> MKNPSFDWERLKDVFYRSRAIGELKWPTQYEEFKCALSLTVIAVEIQDFIQVYNYFGQLLGKINLQRIHEDIIKFEFDKDEKLILVTKSSIKIVKGWSPLTIESVPLQDPTIDTIWDYHNGIMLLAKSRDIYKLNGNEWEL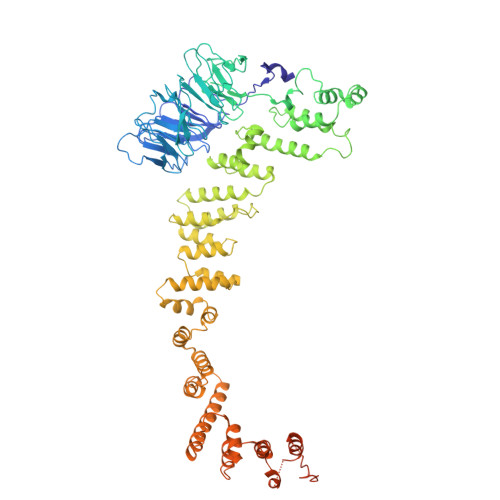LYENKDKKYNLLTKNHWSCNDDSIILLDVDHVYQVSTSNGALLKLITDSSWHKVTISSRGFICLYNMKDNKLQIFRDPARILMEHNLDSTPDDICWCGNDTVACSFEDEIKLYGPDGLYVTFWYPFTVTNLRAEVDGLKVITTEKIYFLSRVQPQTSNIFRIGSTEPGAMLVDSFSLLEDHAPKAIEILKNFVLEKGVLDCIAAAIDEFEPKLQKMLLNAASYGKASLQYKSFDASIFVNACNTIKLLNCFRSFGIFLTVEEYRCISLKGVIDRLLKYHRYYECIQICKLANERFLLGYVFTEWAKDKIKGSPDMEDDELLDKIKSRLSVIDMTDTLQMVAVAKVAYLEGRFQLSRNLALLEKNEEARIEQLYNLDDDSIALKECIKVQNYSLTISLLIALSKKLTNSQLTKLLIIDMFNNPLYLYYMRMDKAYLYDFYRQTDRFIDLAHVLLQQGKEQQSLHSFLPQIKDLYSQVQNSEVVNNTIEQLQRQEKLWIYQESLGKRFAISFTNMTLDQTLSKLIETGQDKQVKEIVKKFKISEKKLYHLKCKTLVEAKKFDELLQFAQSRKSPIGYMPFYTYLKSRGHMDKASPYVNMIPGLSYQEKKKLYVECRGFRDAIQLAGKEKDIPGLKEIYNIIPPNEPELKALANETMSRI(2S,3R,4S,5R,6R)-6-[[[(2R,3S,4R,5R)-5-(2,4-dioxopyrimidin-1-yl)-3,4-dihydroxy-oxolan-2-yl]methoxy-hydroxy-phosphoryl]oxy-hydroxy-phosphoryl]oxy-3,4,5-trihydroxy-oxane-2-carboxylic acid | C15 H22 N2 O18 P2 | 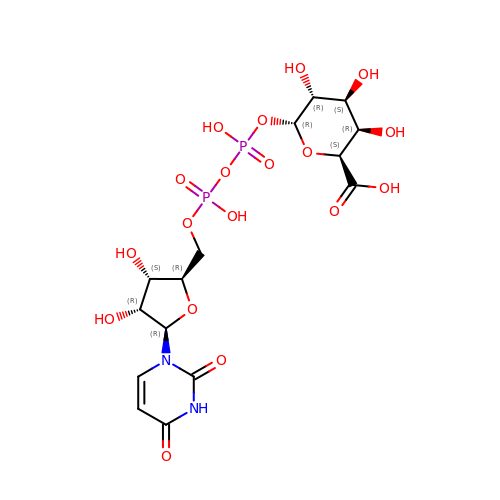HDYANYHVCAPMJV-GXNRKQDOSA-N>MAHHHHHHMSLNVEAAHPFIAARIHGLDLSKPLSDERIVEIEQASGQYPVLIFPRQYIDDDQLLAFAAGFGPLQVAVSYSTRPEDHRLAPMINDISNLSKENQTYRPGDRRRMNNLTSRRWHSDASYLPLPARYSFLLSYIVPAVGGQTQFADMRAAYDKLPDHLRKVVEGLSCHYDIMASRAAAGFYDASDEERKALAPCIHELVRTHPISGRKSLYLSSHATHVVGWPEPEGRDLLRELTEFATQPQFVYSHEWSVRDLVMWDNRALMHRG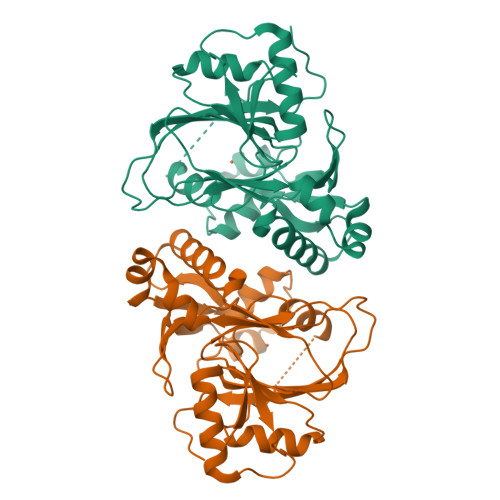RPHIPETDVREMHRATTLDDRTWTRGSNQPVAASVA[4x]>GGKLSEHLRYCDSILREMLSKKHAAYAWPFYKPVDAEALELHDYHDIIKHPMDLSTVKRKMDGREYPDAQ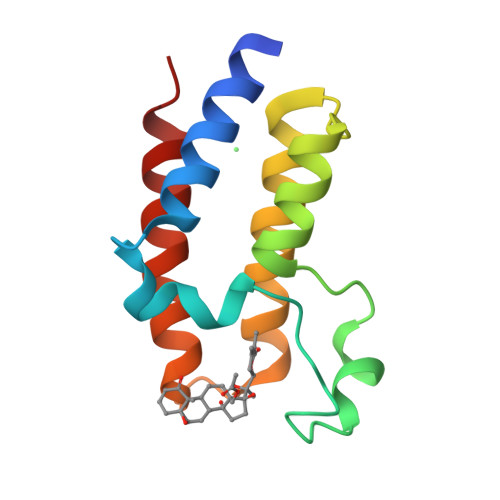GFAADVRLMFSNCYKYNPPDHEVVAMARKLQDVFEMRFAKMP[11x]> AVANSIVSSVAPGKEPGSLVCIQAKDGKVIGMGARVHCGPATVLVTAGHVLKKGMIADLYLAKYSVSSKEGKRVLMDPTW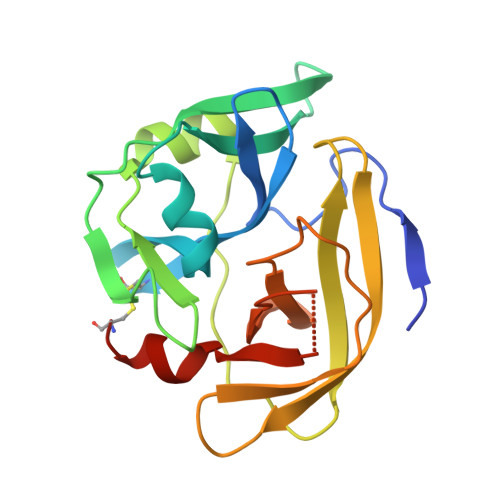KIEYGSLNKEADVISVQVPAAVWSRLGVTAARVRKPTVKVPVLAYGGEASGLLQSSQGFATPDGNMSVAHSCSTRPGWAGTPLYAGSDIVAIHRRWEDIGVKNLATNLSIFHANCESSE>[2x]MASDYEAVNTNPYGVSDGELGPLKYGARFMNMQQRVIPIGSPSLTTGPGNDLQNTDLISSGNYIGYFGNNNNWGFNNEANWNFTDSRMNYAYQNFYSQIFLPWNEIYEIAKDSDSPSEQAILEIANIVRNIAWLRATDVFGPIAYNSAGDGSIAPKFDSQEVVYRSMLADLSKSVELLNTISYSVMAQYDLIYNGNVQNWVKLANSLMLRIVVRVHFIDETLAKEYITKALDPKNGGVIEDISSEAKIKSSDKMPLLNSMLASVNEYN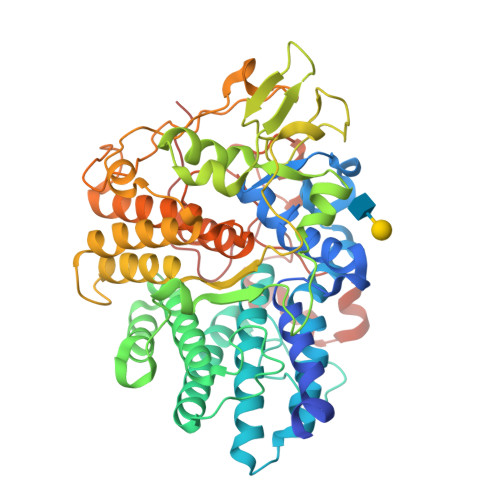ETRMGATIWGYLDGYKDPRLSAYFTEGTYGSGSWAQTGYFPVAPTNSKSKSETSYSAKFASRPKVDSNSPLYWFRASETYFLKAEAALYNLIGGDPKTFYEQGINISFQEQGVSGVATYLSGTGKPTGLTGSNYKYGTYNHDLSIGNTSPKWDDYTGNLSKQEEQLQKIITQKYLALYPNAVEAWTEYRRTGFPYLMKPMDEAAPGRIGASIEDCRVPERFRFAPTAYNSNPNMAEIPTLLGGGDIGATKLWWVRSNRPKQPNQ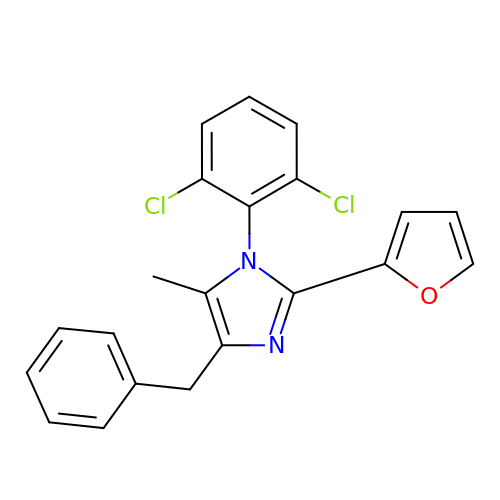1-[2,6-bis(chloranyl)phenyl]-2-(furan-2-yl)-5-methyl-4-(phenylmethyl)imidazole | C21 H16 Cl2 N2 O | YQPVLABIYDUDBN-UHFFFAOYSA-N>SNAIRPTIGQQMETGDQRFGDLVFRQLAPNVWQHTSYLDMPGFGAVASNGLIVRDGGRVLLVDTAWTDDQTAQILNWIKQEINLPVALAVVTHAHQDKMGGMDALHAAGIATYANALSNQLAPQEGLVAAQHSLTFAANGWVEPATAPNFGPLKV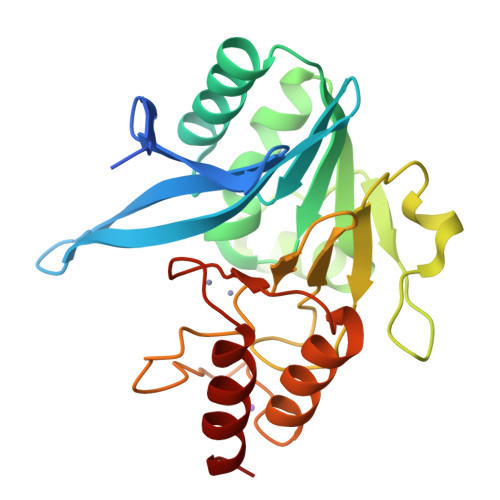FYPGPGHTSDNITVGIDGTDIAFGGCLIKDSKAKSLGNLGDADTEHYAASARAFGAAFPKASMIVMSHSAPDSRAAITHTARMADKLR[4x]Members of the KDM5 (also known as JARID1) sub-family are 2-oxoglutarate (2-OG) and Fe2+-dependent oxygenases acting as histone 3 lysine 4 trimethyl (H3K4me3) demethylases, regulating proliferation, stem cell self-renewal, and differentiation. Members of the KDM5 sub-family of JmjC-KDMs are transcriptional co-repressors, which specifically catalyze the removal of all possible methylation states from lysine 4 of histone H3 (H3K4me3/me2/me1), with highest activity found toward H3K4me3. The KDM5 family and domain architecture is conserved from yeast to humans, displaying a similar pattern with a Jumonji N domain (JmjN), a DNA binding ARID domain (AT-rich interactive domain), a catalytic JmjC, a C5HC2 zinc-finger motif located C-terminally to the JmjC, a PLU-1 motif, as well as one to three methyl-lysine or methyl-arginine binding plant homeodomains (PHDs) denoted PHD-1, PHD-2, and PHD-3. KDM5B plays an important role in stem cell biology by blocking differentiation in embryonic and hematopoietic stem cells (Cellot et al., 2013, Dey et al., 2008).

KDOAM-25 was crystallized in a JmjN-JmjC-linked construct of KDM5B (Johansson et al., 2016). The shift of Y425 creates a cavity which is occupied by a water molecule. The propensity for Y425 to adopt this alternative pose in KDM5B may explain why KDOAM-25 is selective for KDM5 enzymes versus other KDMs that either form different H-bonds to the 4-carboxypyridines (KDM2/3/6/7) or have a less mobile homologous tyrosine (KDM4). The amides KDOAM-25, -28, and -29 were synthesized, and KDOAM-25 was shown to be the most potent of the series with a KDM5B half maximal inhibitory concentration (IC50) of 19 nM and improved selectivity over KDM4C. The experiment indicated that the compound acts a partial competitor of the co-substrate 2-OG, with IC50 values increasing from 27 nM at 4 μM 2-OG, up to 558 nM at 300 μM 2-OG. KDOAM-25 was selective for the KDM5 sub-family with no inhibition below 4.8 μM for any of the other 2-OG oxygenases. As control we used a structurally related inactive compound, KDOAM-32, which is unable to coordinate the catalytic iron in the KDM5 active sites. Structure-based design was used to generate KDOAM-25 without the need for the previously reported ester pro-drugs. KDOAM-25 is a highly selective inhibitor of the KDM5 sub-family of histone lysine demethylases with strongest activity found against the catalytic domain of KDM5B.

> SMFLPPPECPVFEPSWEEFADPFAFIHKIRPIAEQTGICKVRPPPDWQPPFACDVDKLHFTPRIQRLNELEAQTRVKLGGGGARDYTLRTFGEMADAFKSDYFNMPVHMVPTELVEKEFWRLVSTIEEDVTVEYGADIASKEFGSGFPVRDGKIKLSPEEEEYLDSGWNLNNMPVMEQSVLAHITADICGMKLPWLYVGMCFSSFCWHIEDHWSYSINYLHWGEPKTWYGVPGYAAEQLENVMKKLAPELFVSQPDLLHQLVTIMNPNTLMTHEVPVYRTNQCAGEFVITFPRAYHSGFNQGFNFAEAVNFCTVDWLPLGRQCVEHYRLLHRYCVFSHDEMICKMASKADVLDVVVASTVQKDMAIMIEDEKALRETVRKLGVIDSERMDFELLPDDERQCVKCKTTCFMSAISCSCKPGLLVCLHHVKELCSCPPYKYKLRYRYTLDDLYPMMNALKLRAESYNEWALNVNEALEAKINK> MNHKVHHHHHHIEGRVQALFNEISADAVFVTYDGQNIKKYGTHLDRAKTAYIPASTFKIANALIGLENHKATSTE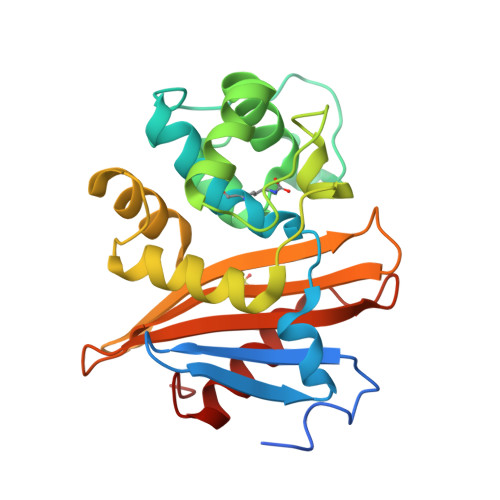IFKWDGKPRFFKAWDKDFTLGEAMQASTVPVYQELARRIGPSLMQSELQRIGYGNMQIGTEVDQFWLKGPLTITPIQEVKFVYDLAQGQLPFKPEVQQQVKEMLYVERRGENRLYAKSGWGMAVDPQVGWYVGFVEKADGQVVAFALNMQMKAGDDIALRKQLSLDVLDKLGVFHYL> LSLKGKKLDFFGRGDTYVSLIDTIPELSRFTACIDLVFMDDNSRYWMAFSYITNNALLGREDIDLG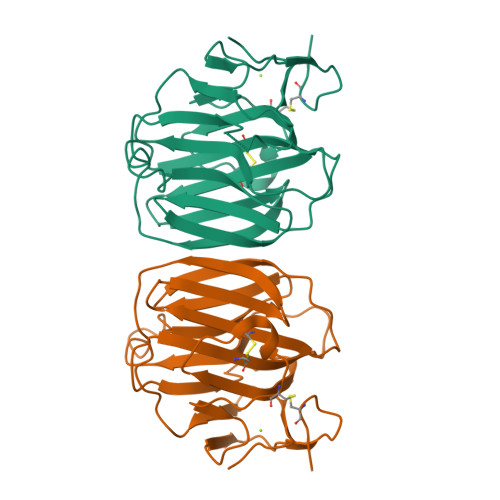LAGDHQQLILYRLGKTFSIRHHLASFQWHTICLIWDGVKGKLELFLNKERILEVTDQPHNLTPHGTLFLGHFLKNESSEVKSMMRSFPGSLYYFQLWDHILENEEFMKCLDGNIVSWEEDVWLVNKIIPTVDRTLRCFVPENMTIQEKSGGGGAGGGGGTDDDDKWSHPQFEK>[3x]SNADLKLDDLKSLTAGSGQQEIEQTINKYSNMLTSIVSSLQEDERGGSAITVHDVGGKKSQYLEKINEVIRRAWAVPTHGHEL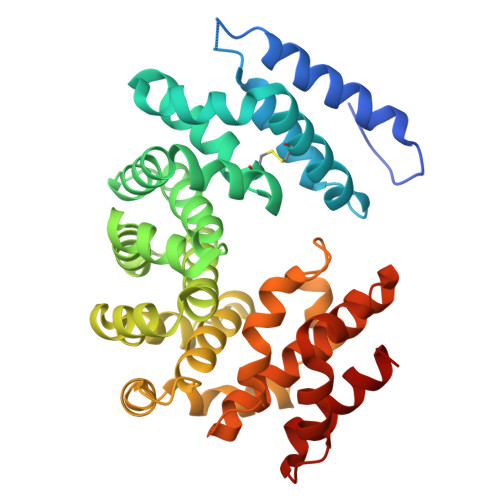GYSLCNSLRQSGGLDLLMKNCVKPDLQFSSAQLLEQCLTTENRKHVVDNGLDKVVNVACVCTKNSNMEHSRVGTGILEHLFKHSEGTCSDVIRLGGLDAVLFECRTSDLETLRHCASALANLSLYGGAENQEEMILRKVPMWLFPLAFHNDDNIKYYACLAIAVLVANKEIEAEVLKSGCLDLVEPFVTSHDPSAFARSNLAHAHGQSKHWLKRLVPVLSSNREEARNLAAFHFCMEAGIKREQGNTDIFREINAIEALKNVASCPNAIASKFAAQALRLIGET>[4x]MRVLALSAVFLVASIIGMPAVAKEWQENKSWNAHFTEH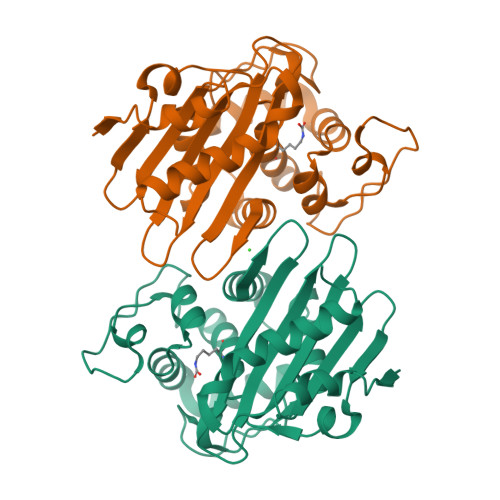KSQGVVVLWNENKQQGFTNNLKRANQAFLPASTFKIPNSLIALDLGVVKDEHQVFKWDGQTRDIATWNRDHNLITAMKYSVVPVYQYFARQIGEARMSKMLHAFDYGNEDISGNVDSFWLDGGIRISATEQISFLRKLYHNKLHVSERSQRIVKQAMLTEANGDYIIRAKTGYSTRIEPKIGWWVGWVELDDNVWFFAMNMDMPTSDGLGLRQAITKEVLKQEKIIP N-({4-[(3-cyclopropyl-1H-pyrazol-5-yl)amino]pyrrolo[2,1-f][1,2,4]triazin-2-yl}methyl)-6-fluoropyridine-3-carboxamide | C19 H17 F N8 O | 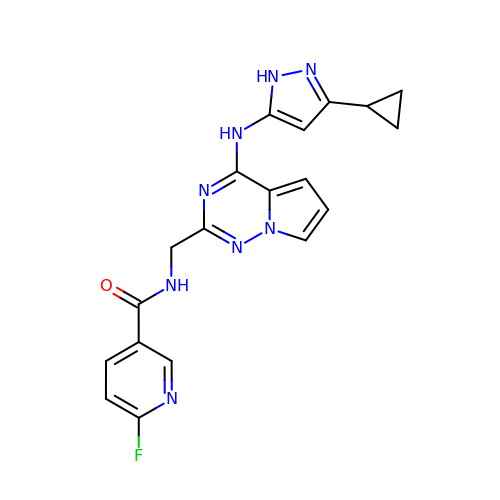FQECDJFBKXFTIW-UHFFFAOYSA-N Transcription of the HIV-1 proviral DNA is initiated by RNA polymerase II (Pol II) binding to the HIV promoter, but stalls after a 30–50 nucleotide transcript containing the trans-activation response region (TAR) is formed. Release of the stalled Pol II is dependent on the recruitment of the host super elongation complex (SEC) to the nascent TAR by HIV-1 trans-activator protein (Tat), a central driver of proviral transcriptional activation. The SEC is assembled on the AFF1 or AFF4 scaffold protein that interacts through small binding domains with the positive elongation factor b (P-TEFb), composed of CDK9 and Cyclin T1 (CycT1), the transcription factor ELL1/ELL2, and ENL/AF9. P-TEFb facilitates promoter escape by phosphorylating two negative elongation factors (DSIF and NELF) as well as the C-terminal domain of Pol II.

To clearly define the interactions between TAR and Tat:P-TEFb, and to determine if direct interactions existed between TAR and AFF4, we solved the crystal structure of the TAR:Tat:SEC complex at 5.9 Å resolution. The structure of TAR bound to Tat:AFF4:P-TEFb reveals extensive interactions between the TAR loop and a composite protein interaction site, composed of CycT1 TRM and the Tat Zn2+-coordination loop, Tat residues 24–29. TAR loop nucleotides G32 and G33 abut the Tat Zn2+ -coordination loop (24-29) and CycT TRM, residues 259-261. The backbone phosphates of nucleotides 30–32 contact basic residues in the CycT TRM region. The structure of the TAR complex with Tat:AFF4:P-TEFb shows no direct contacts between AFF4 and TAR. Instead, AFF4 helix α2 and its N-terminal loop connection to helix α1 are interacting with CycT1 TRM and Tat helix α1. The interaction network between these three protein regions most likely stabilizes the protein interaction surface for TAR and indirectly increases Tat:SEC affinity for TAR in the presence of AFF4. However, there is not interpretable electron density present for residues in the Tat ARM region at the limited resolution of this crystal structure. From there, the ARM (residues 49-57) extends into the major groove of TAR stretching from the TAR bulge towards the phosphate backbone opposite the bulge.

> MAKQYDSVECPFCDEVSKYEKLAKIGQGTFGEVFKARHRKTGQKVALKKVLMENEKEGFPITALREIKILQLLKHENVVNLIEICRTKASPYNRCKGSIYLVFDFCEHDLAGLLSNVLVKFTLSEIKRVMQMLLNGLYYIHRNKILHRDMKAANVLITRDGVLKLADFGLARAFSLAKNSQPNRYTNRVVTLWYRPPELLLGERDYGPPIDLWGAGCIMAEMWTRSPIMQGNTEQHQLALISQLCGSITPEVWPNVDNYELYEKLELVKGQKRKVKDRLKAYVRDPYALDLIDKLLVLDPAQRIDSDDALNHDFFWSDPMPSDLKGMLST;> MEGERKNNNKRWYFTREQLENSPSRRFGVDPDKELSYRQQAANLLQDMGQRLNVSQLTINTAIVYMHRFYMIQSFTQFPGNSVAPAALFLAAKVEEQPKKLEHVIKVAHTCLHPQESLPDTRSEAYLQQVQDLVILESIILQTLGFELTIDHPHTHVVKCTQLVRASKDLAQTSYFMATNSLHLTTFSLQYTPPVVACVCIHLACKWSNWEIPVSTDGKHWWEYVDATVTLELLDELTHEFLQILEKTPNRLKRIWNWRACEAA;> SPLFAEPYKVTSKEDKLSSRIQSMLGNYDEMKDFIG;> XMEPVDPRLEPWKHPGSQPKTACTNCYCKKCCFHCQVCFITKALGISYGRKKRRQRRR> GPLGSMAFLAQLGALADDLVSAIVGIPEDQTTQRDACRDFVLRSLRHHNFGRTNQFEVQDRLN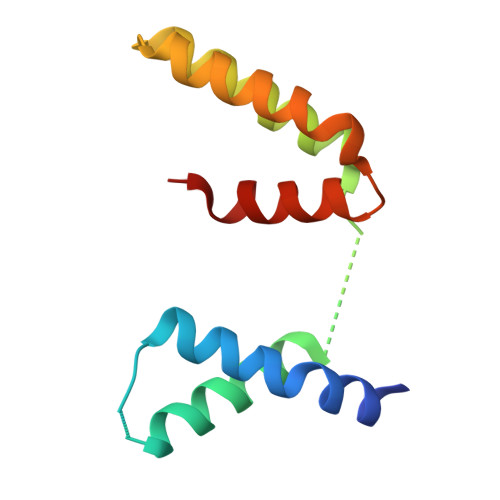GLEERFSIVGRDALADALRTRLDALEPHQNQFTPELLHLLLELADQ> MSFATSITCVLFYMLQLSLLLRGALCISYRALKSAAAAPVAAAGVSAASSRLGGAWEGSIERAEALENLSNEVFGRGN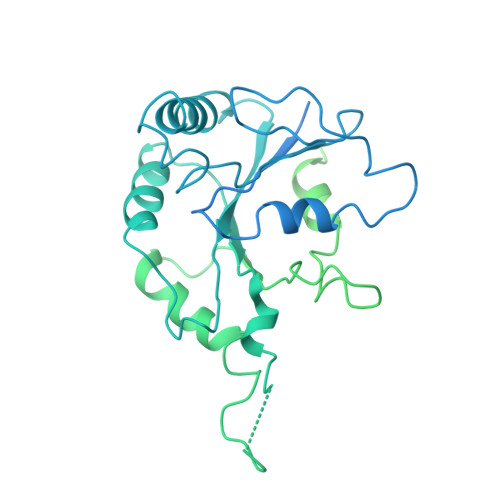RHLKNVETLTALPEGLHSFPEVCFIGKPGCGKSSLISCLLHNHRLGKAGATAGTTRLLQFFNVGDALLLVDTPGYGGWRGREVGQRLAEQANAFSILFRYLALRNGSNLKRVYWLMESSAPTPVSFQPRDEELLTFLSRERIPFSVVLTKIDRHWRHYAEQQRTADRVGNDGFVHPRHRRPETHDQGFFTRTSLPQDGVARNMQEVYEFLGTDQVPILGVSANRLQPNRSRNLELLQHDIVHYCTQDLLHSEELSFRNMHKLSYAPPTADRIHEIQLRYPVESFVVPENNNMSLARMVEHHEEMKARFCENNVCARRLSAKDVAACHLESVAKLKAACKHDTAERERAEKVRPTATYLFESTLAAAVTSLPLPGDVAGLLRASEAQGTATASVSRVGGLPERWKECDDHNAEACAADVCASRRFRVRPLLVGERQTSRDSLGDILERALDEEEPRQDFAGSIVDKGEKTANAASPPHCAHAETTSSSHTLNPVPDEAPVPQPYRVDAVLLQEQPLEALPLPAMLDPDAHYVTAIDGTPIPRSMISVSVEQLAVSKDDELAHFATKSGAGAYEELIVADQEKSNAGADLFMETSDVAHLPEEVQTQLEEACARLTRSAARKQKERFLTKYVERKRKERSIYMQAEGYMCPWLGRSEGRSVVQGFAGSCGTGKGGAVMRDLKQKGFGGKSYSARTMKNRGRATKKTGFWAA> KIL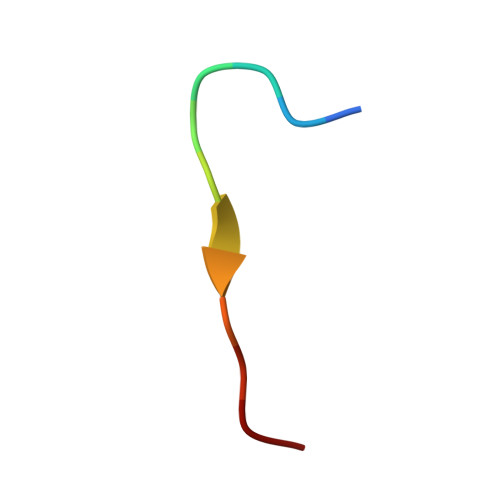LTPRRRQRL>[2x]MATQTSKNPESVHDFTVKDAKENDVDLSIFKGKVLLIVNVASKCGMTNSNYAEMNQLYEKYKDQGLEILAFPCNQFGEEEPGTNDQIT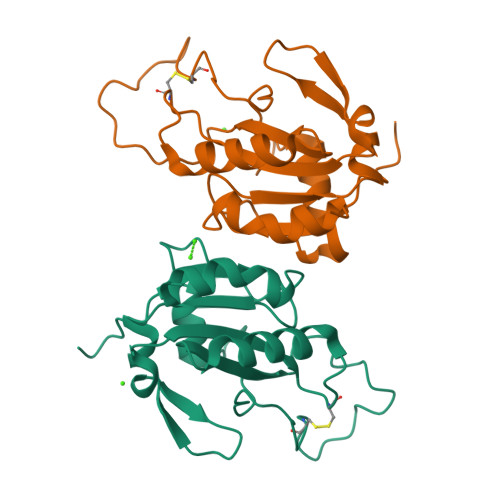DFVCTRFKSEFPIFDKIDVNGENASPLYRFLKLGKWGIFGDDIQWNFAKFLVNKDGQVVDRYYPTTSPLSLERDIKQLLEIS> MLRWLIGGGREPQGLAEKSPLQTIGEEQTQNPYTELLVLKAHHDIVRFLVQLDDYRFASAGDDGIVVVWNAQTGEKLLELNGHTQKITAIIT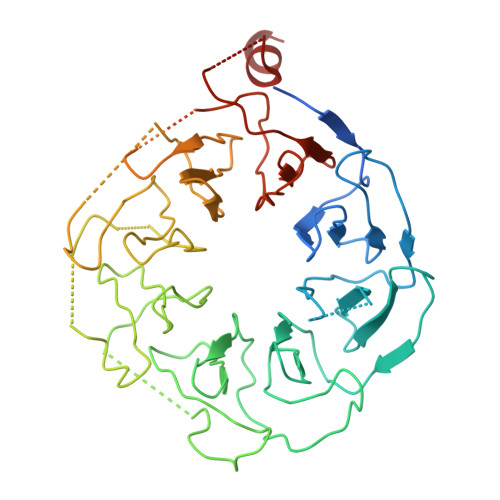FPSLESCEEKNQLILTASADRTVIVWDGDTTRQVQRISCFQSTVKCLTVLQRLDVWLSGGNDLCVWNRKLDLLCKTSHLSDTGISALVEIPKNCVVAAVGKELIIFRLVAPTEGSLEWDILEVKRLLDHQDNILSLINVNDLSFVTGSHVGELIIWDALDWTMQAYERNFWDPSPQLDTQQEIKLCQKSNDISIHHFTCDEENVFAAVGRGLYVYSLQMKRVIACQKTAHDSNVLHVARLPNRQLISCSEDGSVRIWELREKQQLAAEPVPTGFFNMWGFGRVSKQASQPVKKQQENATSCSLELIGDLIGHSSSVEMFLYFEDHGLVTCSADHLIILWKNGERESGLRSLRLFQKLEENGDLYLAV> GPLGSMASLMEVRDMLALQG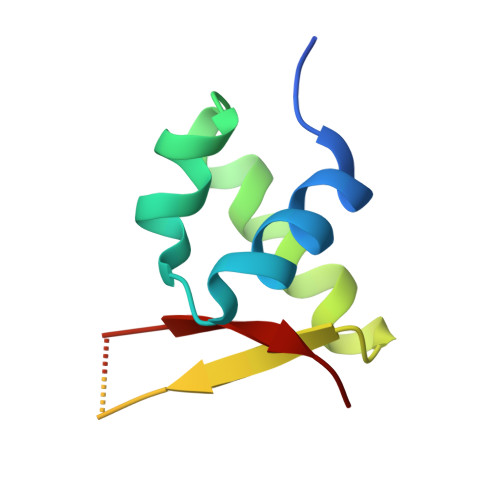RMEAKQLSARLQTPQPLIDAMLERMEAMGKVVRISETSEGCLSGSCKSCPEGKAACRQEWWALRL Non-homologous end joining (NHEJ) is a major pathway for detection and repair of DSBs in mammalian cells. Here we perform systematic interactome analyses of human NHEJ factors and identify a novel XRCC4-like protein named paralogue of XRCC4 and XLF (PAXX). The crystal structure study reveals that PAXX forms a homodimer through its N-terminal domain that is structurally similar to XRCC4 and XLF. Thus, our data reveal that PAXX is a new core NHEJ factor that plays a key role in the organization of NHEJ complexes for the repair of diverse types of DSB ends.

Immunoblotting of the Ku80-associated complex further validated this finding. Based on the sequence and structural similarity to XRCC4 and XLF (see below), we renamed C9orf142 as PAXX. The space groups for both data sets were P6522, with two molecules in each asymmetric unit. Seven β-strands (S1–S7) and three helixes (H1–H3) were observed in the PAXX 1–145 structure, in which a globular head domain and a coiled-coil stalk formed a dimer, consistent with the observation that PAXX 1–145 exists primarily as a dimer in solution. As predicted, the N-terminal domain of PAXX was highly similar to those of XLF and XRCC4. Compared with XLF, PAXX showed more structural similarities to XRCC4. In XRCC4 and PAXX, the angle between the head domain and H3 is only ~45° due to a lack of tension. Structurally, the N-terminal domain of PAXX is more similar to that of XRCC4, as both exhibit a 45° angle between the head domain and the helix stalk. In addition, compared with XRCC4 and XLF, PAXX has a much shorter coiled-coil stalk. The extended stalk of XRCC4 is required for Lig4 binding, implicating that the N-terminal domain of PAXX may lack the ability to bind Lig4. We generated a combined mutation (Nmut: L96D, L98D, L105D and L109D) in this region of PAXX, which is expected to disrupt the hydrophobic interface.

>[2x]MGSSHHHHHHSQGSEFMDPLSPPLCTLPPGPEPPRFVCYCEGEESGEGDRGGFNLYVTDAAELWSTCFTPDSLAALKARFGLSAAEDITPRFRAACEQQAVALTLQEDRASLTLSGGPSALAFDLSKVPGPEAAPRLRALTLGLAKRVWSLERRLAAAEET>[4x]MSLILESLVTTLDEQGRINLAPLGPIVLPPQSPGGLPQFLLRPYEGSTTCDNLLASGNAVIHVIDDALLIAKTAIGKVDASDLVVPIPGLEDTHVRLKRCHRWFAVRVTQRA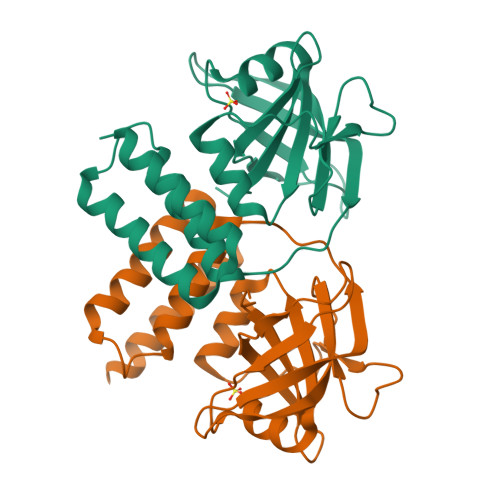GTPPRHELTARCLASGLVDPFFGFNRAKHAVIEAAVAATRLHLLPPEEIEEELERARIAIEKTGGEPEREALQLIRRHVRESSISEGHHHHHH>MPSDIEIARAATLKPIAQVAEKLGIPDEALHNYGKHIAKIDHDFIASLEGKPEGKLVLVTAISPTPAGEGKTTTTVGLGDALNRIGKRAVMCLREPSLGPCFGMKGGAAGGGKAQVVPMEQINLHFTGDFHAITSAHSLAAALIDNHIYWANELNIDVRRIHWRRVVDMNDRALRAINQSLGGVANGFPREDGFDITVASEVMAVFCLAKNLADLEERLGRIVIAETRDRKPVTLADVKATGAMTVLLKDALQPNLVQTLEGNPALIHGGPFANIAHGCNSVIATRTGLRLADYTVTEAGFGADLGAEKFIDIKCRQTGLKPSSVVIVATIRALKMHGGVNKKDLQAENLDALEKGFANLERHVNNVRSFGLPVVVGVNHFFQDTDAEHARLKELCRDRLQVEAITCKHWAEGGAGAEALAQAVVKLAEGEQKPLTFAYETETKITDKIKAIATKLYGAADIQIESKAATKLAGFEKDGYGKLPVCMAKTQYSFSTDPTLMGAPSGHLVSVRDVRLSAGAGFVVVICGEIMTMPGLPKVPAADTIRLDANGQIDGLFAAAL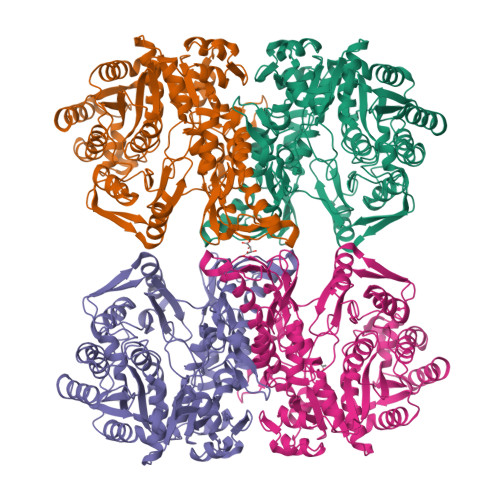EHHHHHH[8x]> NSIALKNNTLWTGPKPEANCIIEYGKQNPDSKLTLILVKNGGIVNGYVTLMGASDYVNTLFKN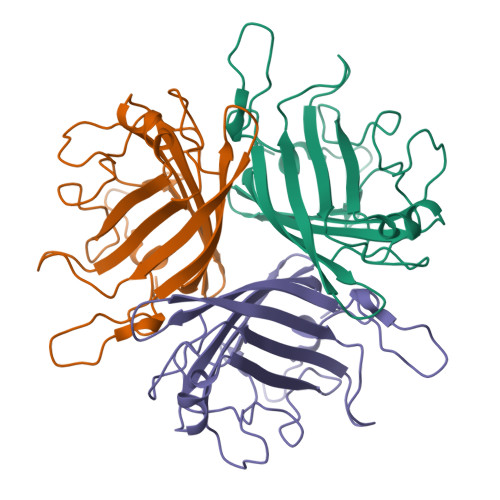KNVSINVELYFDATGHILPDSSSLKTDLELKYKQTADFSARGFMPSTTAYPFDLPNAGTHNENYIFGQCYYKASDGALFPLEVTVMLNKRLPDSRTSYVMTFLWSLNAGLAPETTQATLITSPFTFSYIREDD> MTTYLEFIQQNEERDGVRFSWNVWPSSRLEATRMVVPVAALFTPLKERPDLPPIQYEPVLCSRTTCRAVLNPLCQVDYRAKLWACNFCYQRNQFPPSYAGISELNQPAELLPQFSSIEYVVLRGPQMPLIFLYVVDTCMEDEDLQALKESMQMSLSLLPPTALVGLITFGRMVQVHELGCEGISKSYVFRGTKDLSAKQLQEMLGLSKVPLTQATRGPQVQQPPPSNRFLQPVQKIDMNLTDLLGELQRDPWPVPQGKRPLRSSGVALSIAVGLLECTFPNTGARIMMFIGGPATQGPGMVVGDELKTPIRSWHDIDKDNAKYVKKGTKHFEALANRAATTGHVIDIYACALDQTGLLEMKCCPNLTGGYMVMGDSFNTSLFKQTFQRVFTKDMHGQFKMGFGGTLEIKTSREIKISGAIGPCVSLNSKGPCVSENEIGTGGTCQWKICGLSPTTTLAIYFEVVNQHNAPIPQGGRGAIQFVTQYQHSSGQRRIRVTTIARNWADAQTQIQNIAASFDQEAAAILMARLAIYRAETEEGPDVLRWLDRQLIRLCQKFGEYHKDDPSSFRFSETFSLYPQFMFHLRRSSFLQVFNNSPDESSYYRHHFMRQDLTQSLIMIQPILYAYSFSGPPEPVLLDSSSILADRILLMDTFFQILIYHGETIAQWRKSGYQDMPEYENFRHLLQAPVDDAQEILHSRFPMPRYIDTEHGGSQARFLLSKVNPSQTHNNMYAWGQESGAPILTDDVSLQVFMDHLKKLAVSSA;> EGLRVVNLLQERNMLPSTPLKPPVPNLHEDIQKLNCNPELFRCTLTSIPQTQALLNKAKLPLGLLLHPFKDLVQLPVVTSSTIVRCRSCRTYINPFVSFLDQRRWKCNLCYRVNDVPEEFLYNPLTRVYGEPHRRPEVQNATIEFMAPSEYMLRPPQPPVYLFVFDVSHNAVETGYLNSVCQSLLDNLDLLPGNTRTKIGFITFDSTIHFYGLQESLSQPQMLIVSDIEDVFIPMPENLLVNLNESKELVQDLLKTLPQMFTKTLETQSALGPALQAAFKLMSPTGGRMSVFQTQLPTLGVGALKPREEPNHRSSAKDIHMTPSTDFYKKLALDCSGQQVAVDLFLLSGQYSDLASLGCISRYSAGSVYYYPSYHHQHNPVQVQKLQKELQRYLTRKIGFEAVMRIRCTKGLSIHTFHGNFFVRSTDLLSLPNVNPDAGYAVQMSVEESLTDTQLVSFQSALLYTSSKGERRIRVHTLCLPVVSTLNDVFLGADVQAISGLLANMAVDRSMTASLSDARDALVNAVIDSLSAYRSSVLSNQQPGLMVPFSLRLFPLFVLALLKQKSFQTGTNARLDERIFAMCQVKNQPLVYLMLTTHPSLYRVDNLSDEGALNISDRTIPQPPILQLSVEKLSRDGAFLMDAGSVLMLWVGKNCTQNFLSQVLGVQNYASIPQPMTDLPELDTPESARIIAFISWLREQRPFFPILYVIADESPMKANFLQNMIEDRTESALSYYEFLLHIQQQVNK;> MVLLTMIARVADGLPLAASMQEDEQSGRDLQQYQSQAKQLFRKLNEQSPTRCTLEAGAMTFHYIIEQGVCYLVLCEAAFPKKLAFAYLEDLHSEFDEQHGKKVPTVSRPYSFIEFDTFIQKTKKLYIDSRARRNLGSINTELQDVQRIMVANIEEVL;> EVTSSV

The packaging of cargo transmembrane proteins into COPII-coated vesicles entails a direct interaction between COPII protein and cytoplasmically-oriented ER export signals. About a half dozen export signals have been identified to date, almost all comprising short peptide motifs, all of them binding to the Sec24 subunit of the COPII inner coat. The ΦC export signal was identified in studies of p24-family and ERGIC-53 proteins, and comprises a C-terminal signature of a pair of hydrophobic residues or a single terminal valine residue. The ΦC motif contacts a site on Sec24a that is also the binding site for the LxxLE- and DxE-class export motifs (Miller et al., 2003; Mossessova et al., 2003).

A series of ΦC-signal peptides was synthesized, based on a core sequence of yeast Emp24p, and individual peptides were soaked at high concentrations into two crystal forms of human COPII protein: one comprising Sec23a/Sec24a•Sec22b, the other Sec24c. For all ΦC sequences, we observed clear evidence for peptide binding to a site on Sec24a in the Sec23a/Sec24a•Sec22b crystals, based on the presence of residual electron density that matches the peptide sequence (this binding site is occluded in the Sec24c crystals). The finding that multiple classes of export motifs bind to a common site is surprising, but the COPII•ΦC crystal structures highlight that the common molecular feature is carboxylate-group recognition by the clustered arginine residues of the B site—the terminal carboxylate group of the ΦC motif adopts a similar position and bonding arrangement to the carboxylate of the glutamate side chains of LxxLE and DxE motifs (Mancias and Goldberg, 2008; Mossessova et al., 2003). Thus, specific recognition of the ΦC motif involves the terminal carboxylate group bonding to Arg750 and Arg752 of Sec24a, with the penultimate hydrophobic residue of the motif nestling against Tyr496, and the terminal hydrophobic residue fitting to a pocket of hydrophobic side chains.> MFQSILMIVLVVMSISLFVCFIRTLIGPTMSDRIVALD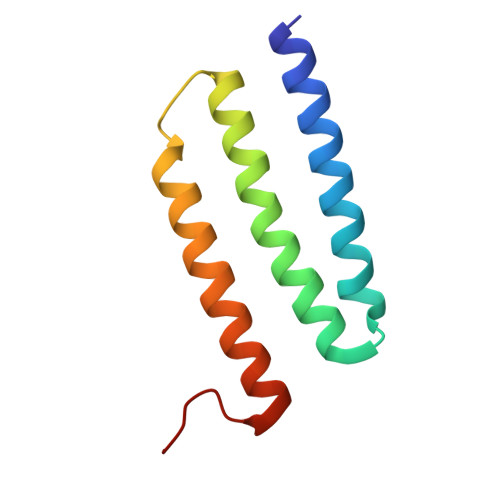TFGINLIGFIGVIMMLQETLAYSEVVLVISILAFIGSIALSKFIERGVVFDRG Triosephosphate isomerase (TPI; EC 5.3.1.1) is a glycolytic enzyme which catalyses a critical step in glycolysis in which a toxic triose dihydroxyacetone phosphate (DHAP; produced by aldolase in the previous step) is reversibly converted to d-glyceraldehyde-3-phosphate (GAP; Rieder & Rose, 1959). The TPI, in most species, is a homodimer with the substrate-binding site located close to the dimer interface. Only the dimeric form of TPI is active, and disruption of the interactions forming the dimer can result in inhibition and inactivation of the enzyme. Triosephosphate isomerase (TPI) is a glycolytic enzyme that has been researched as a drug target for various parasites, including F. hepatica.

In this study, we report the expression, purification and crystallization of FhTPI and its monoclinic structure at 1.51 Å resolution. The asymmetric unit contains two FhTPI dimers. In subunit C, several loops were built with an alternative conformation of the main chain. The main secondary structures of the FhTPI monomer are a single β-sheet (an eight-stranded barrel) and 15 α-helices, which are arranged in a α/β barrel motif. There are 27 hydrogen bonds and seven salt bridges at the dimer interface that stabilize it. Out of these interactions, of especial interest is the interaction of Lys50 and Asp51 that participate in hydrogen-bond and salt-bridge formation at the dimer interface. These two residues do not exist in the mammalian hosts of F. hepatica, where they are substituted by Asp50 and Phe51 as shown by the aligned TPI sequences. As attempts to crystallize FhTPI in complex with the potential inhibitor TCBZ did not yield any diffraction-quality crystals, the structure was used in molecular-docking experiments to locate structural differences between parasitic and mammalian host enzymes, with the aim of developing new parasite-specific inhibitors of glycolysis. In our studies, both the ‘targeted’ and ‘blind’ docking approaches identified TCBZ binding poses in a region within the dimer interface, distant from the catalytic residues.

>MASNRKFFVGGNWKMNGSKESNQKLLKTLSDAKPDANTEILVAVPFVYLKDVREHLDKRFHVAAQNCYKVASGAFTGEISPAMIRDCGCEWVILGHSERRHIFGESDELIGEKVNHALTCGLKVVPCIGEKLDEREAGKTEQVCFRQLDAIKKGIPKAEDWSRVVIAYEPVWAIGTGKTASPEQAQEVHHAVRQWLEKNVSQAVASSLRITYGGSVTAANCKELAKKPDVDGFLVGGASLKPEFVDICNANRG[4x]> MKRKYLKLMIGLALAATLTLSGCSLPGLSAAADQTIKIGAQSMSESEIIASMLGQLIEHHTDLKTTTI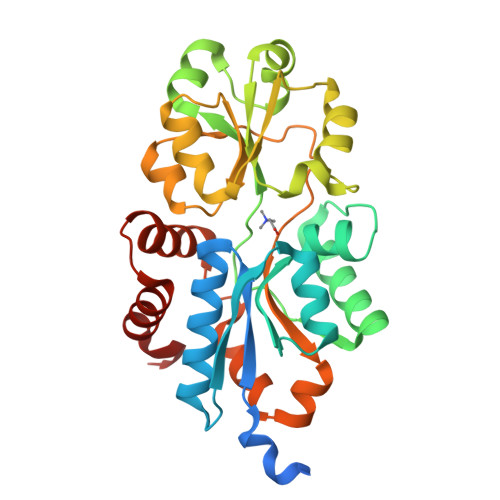KNLGSNAVQQQALMNGEIDIAATRYTGTALTGTLRMEPEKDPDKALALTQREFKKRYDLKWYDSYGFDNTYAFTVSKELADQYHLETVSDVKKWAPQLKLGVDNYWMKLKGNGYQDFTKTYGMTFGGTYPMQIGLVYDAVKSGKMDIVLAYSTDGRIKSYGLKMLKDDKQFFPPYDCSPVVPEKVLKEHPELEGIIKKMLGKIDTATMQELNYEVDGNLKEPSVVAKEYLEKHRYFES Present in the small intestine, cellular retinol binding protein 2 (CRBP2) plays an important role in the uptake, transport, and metabolism of dietary retinoids. All CRBPs share the same protein structure architecture. These small soluble proteins fold into a single β-barrel that shields the central hydrophobic cavity that constitutes a solitary binding site for retinoids. Access to the binding pocket is governed by a “portal region” composed of conformationally flexible loops connecting neighboring β-strands. By examining chemical libraries of bioactive lipids, we provided evidence for the selective interaction of CRBP2 with a subset of nonretinoid ligands with the highest affinity for sn-1 and sn-2 MAGs that contain polyunsaturated C18-C20 acyl chains.

Importantly, an analogous correlation of Kd values was seen for other sn-1 and sn-2 MAG pairs represented by 1-linoleoyl glycerol and 2-linoleoyl glycerol (2-LG) with affinities of 97.1 ± 27.6 and 40.0 ± 4.4 nM, respectively. The comparison of the positions of 2-AG and 2-LG or 2-oleoyl glycerol (2-OG) supports this hypothesis. Despite the two-carbon difference in length, the aliphatic ends of the fatty acid chains for each of these ligands are located exactly in the same place. This spatial length compensation is achieved by the adoption of a more extended configuration by the C18 chains of 2-LG and 2-OG as compared with 2-AG. The main difference is seen in the location of carbon atoms 3–6 of the chains, whereas the portions of the fatty acid moieties that make contact with the portal region of the protein are very similar in these ligands. Thus, the conservation of the interactions of lipids with the portal region seems to be key to the stabilization of the protein configuration in the ligand bound (close) state that macroscopically can be observed as lower Kd. The acyl chains of 2-AG, 2-LG, or 2-OG bent inside the binding pocket making contact with the side chains of the β5-β6 loop, α-helices I and II, and finally the β3-β4 loop at the ends of the carbon chains. In contrast to the lengths of the fatty acid moieties, comparing the positions of MAGs with polyunsaturated and monounsaturated acyls did not indicate differences in the spatial orientation of the ligands in the binding site. Despite the absence of double bonds, the linoleoyl and oleoyl moieties adopted the same kinked configuration as observed for 2-AG.

>MTRDQNGTWEMESNENFEGYMKALDIDFATRKIAVRLTQTKVIDQDGDNFKTKTTSTFRNYDVDFTVGVEFDEYTKSLDNRHVKALVTWEGDVLVCVQKGEKENRGWKQWIEGDKLYLELTCGDQVCRQVFKKKLVPR[2x]> MSAKKIVLKSSDGESFEVEEAVALESQTIAHMVEDDCVDNGVPLPNVTSKILAKVIEYCKRHVEAAASKAEAVEGAATSDDDLKAWDADFMKIDQATLFELILA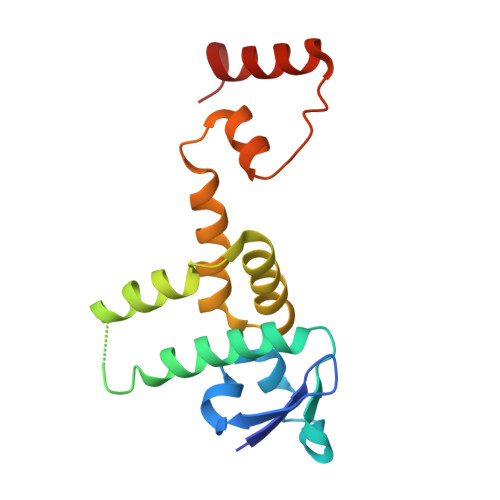ANYLNIKNLLDLTCQTVADMIKGKTPEEIRTTFNIKNDFTPEEEEEVRRENQWAFE>ACUCGUUUGAGCGAGUAUAAACAGUUGGUUAGGCUCAAAGCGGAGAGCAG[2x];>UCUGCUCUC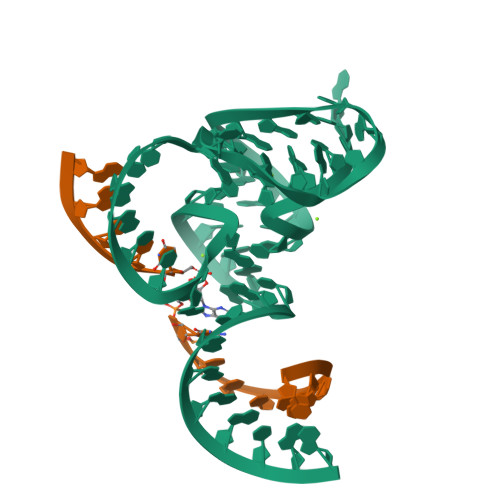XUCCAA[2x]> AMGSLRAASASLILGNRVAERELEVAYSCDGVRAEVIPRMRRVDLYLKHDSQSYKLEVLFEDINECFGCHLDGTGAILLQLTYAPRIHIAISGSTVKSRFTDDRFHACKEDAKFAWVRALDFTPNSSFGECSTLVLKLSKGASVSYILESLPFSGELGELAIASMDVFGSSSNVVPLVDCPNGFSVPYEVLFRLNSLVHMGKLVARHVNADLFKVLEDLSIDTLRRIFEKMSKLKSTCYEPLQFIRHEAHSMNMRKKALSNKRESGKLMRCYRIHITPSKIYCLGPEEEVSNYVVKYHSEYASDFARVTFVDEDWSKLSPNALSARTEQGFFSKPLKTGLYHRILSILKEGFCIGPKKYEFLAFSASQLRGNSVWMFASNSSLTAENIRRWMGHFEDIRSVSKCAARMGQLFSSSRQTFEVSSYDVEVIPDIEVTTDGTKYIFSDGIGKISTRFARQVAKLIGLDPAHPPSAFQIRYGGYKGVITIDPTSFFN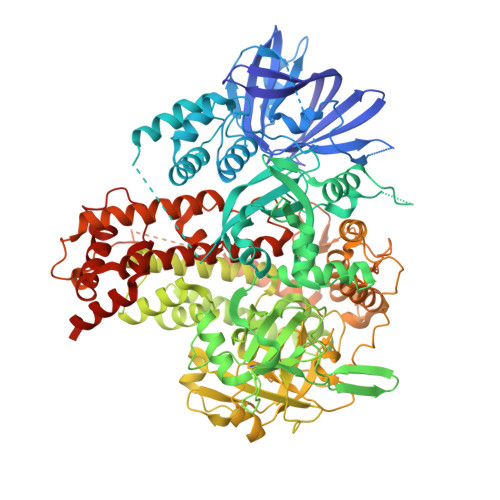LSLRPSMKKFESKSTMLNITNWSKSQPCYVNREIISLLSTLGIKDEVFESMQQDDMHESDGMLTNKEAALSVLGKIGGGDTKTAADMLLQGYEPSSEPYLLMILKAHRANRLTDIRTRCKIHVQKGRVLIGCLDETCKLEYGQVYIRITKNHKEQKYSEQPFFCNDDGKTAVIVGKVAITKNPCLHPGDVRVLEAVYDPGLDARGLIDCVVFPQRGERPHPNECSGGDLDGDLFFITWDDKLIPAAVDAPMDYTATRPRIMDHAVTLEEIQKHFVSYMINDTLGAISTAHLIHADRDPLKARSPECVQLAALHSMAVDFAKTGAPAEMPLALRPREFPDFMERWERPMYVSNGVLGKLYRAALRHAADAAALLPAGPPSCVYDPDLEVAGFDEFLDAAEERYEAYAERLGALMTYYSAEREDEILTGNIRNKLVYLRRDNKRYFEMKDRIIAAVDALHAEVRGWLRACKEDDASRVASAWYHVTYHPDRRGEKRFWSFPWIICDTLLAIKAARRCRKRVEDAAVPMDCDGS>IGVCYGVIGNNLPSRSDVVQLYRSKGINGMRIYFADGQALSALRNSGIGLILDIGNDQLANIAASTSNAASWVQNNVRPYYPAVN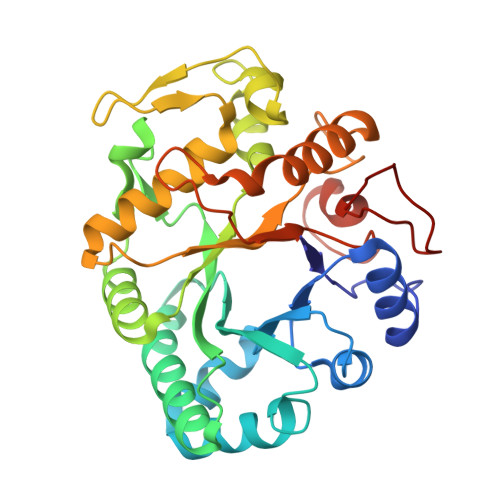IKYIAAGNEVQGGATQSILPAMRNLNAALSAAGLGAIKVSTSIRFDEVANSFPPSAGVFKNAYMTDVARLLASTGAPLLANVYPYFAYRDNPGSISLNYATFQPGTTVRDQNNGLTYTSLFDAMVDAVYAALEKAGAPAVKVVVSESGWPSAGGFAASAGNARTYNQGLINHVGGGTPKKREALETYIFAMFNENQKTGDATERSFGLFNPDKSPAYNIQF[2x]EBNA1 is the viral encoded DNA binding protein essential for the stable maintenance of the EBV circular genome (referred to as episome) during latent infection. EBNA1 binds with high affinity to viral origin of plasmid replication (OriP) to drive latent cycle DNA replication and genome segregation required to maintain stable episome copy number in proliferating cells. EBNA1 is consistently expressed in all EBV-associated tumors, and is thought to provide a survival function in addition to the maintenance of the viral genome. EBNA1 interacts with numerous host proteins important for DNA replication, episome maintenance, and host survival.

To investigate the potential role of amino-acid polymorphisms in the EBNA1 DNA binding domain that may confer NPC risk, we isolated viral DNA from primary EBV positive NPC in patients from Hong Kong. The EBNA1 DBD was amplified by high-fidelity PCR from the HKNPC6-7 variant 2, subcloned, and sequenced. Several polymorphisms were identified that conform to the high-risk forms found in other NPC derived viral strains, including M81 and C666-1. These include 10 amino acid substitutions most of which were considered conservative, but several potential variations that could alter function, including T585I and T502N. We then solved the X-ray crystal structures of NPC and B95-8 EBNA1 DBDs, as well as their co-crystal structures in complex with a cognate DNA binding site derived from EBV OriP. The structures reveal an overall near-identical fold (RMDS of .219 Å) between NPC and B95-8 EBNA1 DBDs. None of the polymorphic amino acids make direct contact with DNA or altered the DNA binding interface. Amino acids A487V, T585I, T502N, D499E, and R594K are on the exposed EBNA1 surface opposite the DNA binding interface, suggesting that they may alter potential interactions of EBNA1 with other proteins. Amino acids T524I, I528V, and L533I are buried within the protein surface and have no apparent effect on overall structure. The NPC- and B95-8 EBNA1 DBDs were next assayed for DNA binding using BIACORE surface plasmon resonance (SPR) assay with two different DNA probes derived from either a single FR site or the paired DS 3+4 binding sites. Both proteins bound with high affinity (16-17 nM for FR, and 11-14 nM for DS 3+4), although NPC-EBNA1 had a slightly reduced affinity for DS 3+4 relative to B95-8 EBNA1 (14.1 vs 11.9 nM).

>RKKGGWFGKHRGQGGSNPKFENIAEGLRVLLARSHVERTTEEGNWVAGVFVYGGSKTSLYNLRRGIALAVPQCRITPLSRLPFGMAPGPGPQPGPLRESIVCYFMVFLQTHIFAEVLKDAIKDLVMIKPAPTCNIKVTVCSFDDGVDLP[2x]> MALPLLNYAPKSQNVRVEGYEIGSEEKPVVFTTENILSSSDMDNLIEAAYRQIFFHAFKWDREKVLES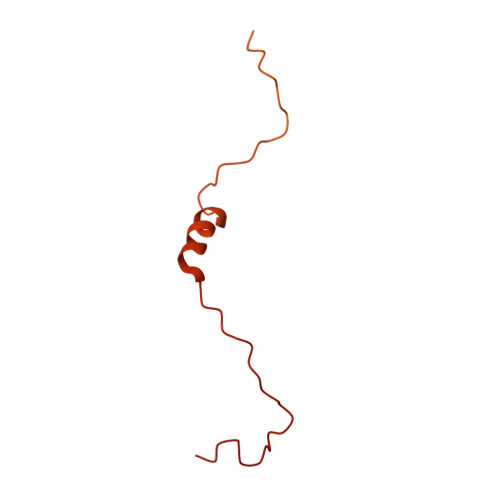QLRNGQITVRDFVRGLLLSNTFRNSFYEKNSNYRFVEHCVQKILGRDVYSEREKIAWSIVVATKGYQGLIDDLLNSDEYLNNFGYDTVPYQRRRNLPGREAGELPFNIKSPRYDAYHRRQLGFPQIVWQNEVRRFIPQEKKLTAGNPMNFLGMARSINPAANTIPKVSAQNINIEASVPRR>GPGSEFRPQPLPPGWERRVDDRRRVYYVDHNTRTTTWQRPTMESVRNFEQWQSQRNQLQGAMQQFNQRYLYSASMLAAENDPYGPLPPGWEKRVDSTDRVYFVNHNTKTTQWEDPRTQGLQNEEPLPEGWEIRYTREGVRYFVDHNTRTTTFKDPRNGKSSVTKGGPQIAYERGFRWKLAHFRYLCQSNALPSHVKINVSRQTLFEDSFQQIMALKPYDLRRRLYVIFRGEEGLDYGGLAREWFFLLSHEVLNPMYCLFEYAGKNNYCLQINPASTINPDHLSYFCFIGRFIAMALFHGKFIDTGFSLPFYKRMLSKKLTIKDLESIDTEFYNSLIWIRDNNIEECGLEMYFSVDMEILGKVTSHDLKLGGSNILVTEENKDEYIGLMTEWRFSRGVQEQTKAFLDG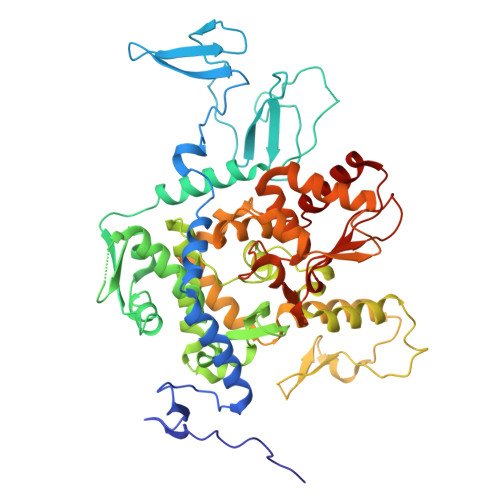FNEVVPLQWLQYFDEKELEVMLCGMQEVDLADWQRNTVYRHYTRNSKQIIWFWQFVKETDNEVRMRLLQFVTGTCRLPLGGFAELMGSNGPQKFCIEKVGKDTWLPRSHTCFNRLDLPPYKSYEQLKEKLLFAIEETEGFGQE[2x]>[2x]AKPDRSSFVPSLFSKKKKNVTMRSIKTTRDRVPTYQYNMNFEKLGKCIIINNKNFDKVTGMGVRNGTDKDAEALFKCFRSLGFDVIVYNDCSCAKMQDLLKKASEEDHTNAACFACILLSHGEENVIYGKDGVTPIKDLTAHFRGDRCKTLLEKPKLFFIQACRGTE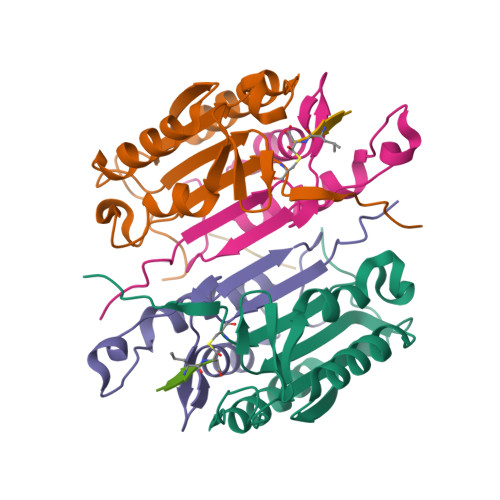LDDGIQ;>[2x]ANPRYKIPVEADFLFAYSTVPGYYSWRSPGRGSWFVQALCSILEEHGKDLEIMQILTRVNDRVARHFESQSDDPHFHEKKQIPCVVSMLTKELYFSQ;> QGHGE>MSALFEPYTLKDVTLRNRIAIPPMCQYMAEDGLINDWHQVHYASMARGGAGLLVVEATAVAPEGRITPGCAGIWSDAHAQAFVPVVQAIKAAGSVPGIQIAHAGRKASANRPWEGDDHIGADDARGWETIAPSAIAFGAHLPNVPRAMTLDDIARVKQDFVDAARRARDAGFEWIELHFAHGYLGQSFFSEHSNKRTDAYGGSFDNRSRFLLETLAAVREVWPENLPLTARFGVLEYDGRDEQTLEESIELARRFKAGGLDLLSVSVGFTIPETNIPWGPAFMGPIAERVRREAKLPVTSAWGFGTPQLAEAALQANQLDLVSVGR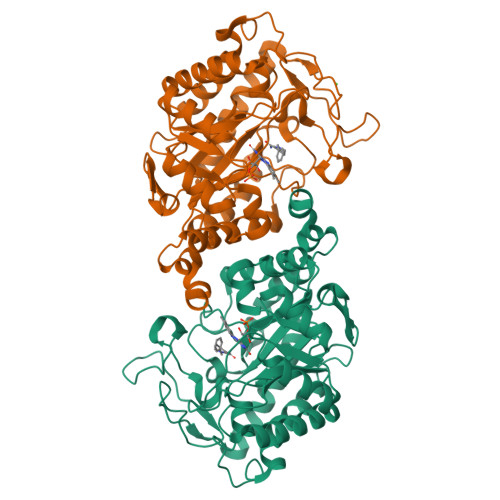AHLADPHWAYFAAKELGVEKASWTLPAPYAHWLERYRRPHHHHHH[2x]> MGSSHHHHHHSSGLVPRGSHMSPSPVPGSQNVPAPAVKKISQYACQRRTTLNNYNQLFTDALDILAENDELRENEGSCLAFMRASSVLKSLPFPITSMKDTEGIPCLGDKVKSIIEGIIEDGESSEAKAVLNDERYKSFKLFTSVFGVGLKTAEKWFRMGFRTLSKIQSDKSLRFTQMQKAGFLYYEDLVSCVNRPEAEAVSMLVKEAVVTFLPDALVTMTGGFRRGKMTGHDVDFLITSPEATEDEEQQLLHKVTDFWKQQGLLLYCDILESTFEKFKQPSRKVDALDHAQKCFLILKLDHGRVHSEKSGQQEGKGWKAIRVDLVMCPYDRRAFALLGWTGSRQFERDL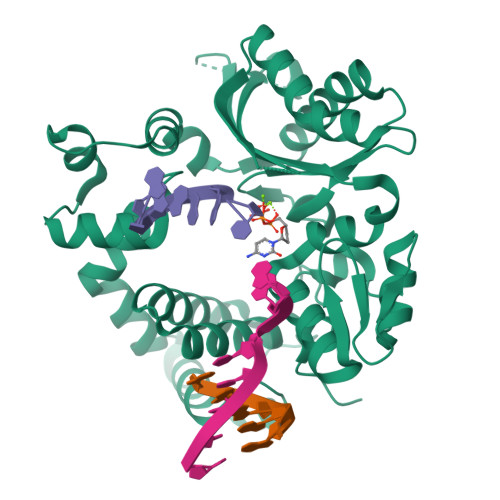RRYATHERKMMLDNHALYDRTKRVFLEAESEEEIFAHLGLDYIEPWERNA> MDIIFVSTGNTCRSPMAEALFKSIAEREGLNVNVRSAGVFASPNGKATPHAVEALFEKHIALNHVSSPLTEELMESADLVLAMTHQHKQIIASQFGRYRDKVFTLKEYVTGSHGDVLDPFGGSIDIYKQ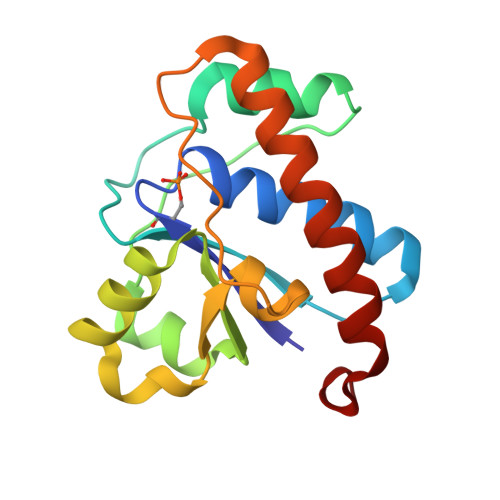TRDELEELLRQLAKQLKKDRRLE4-({6-[(6-chloro-3-{1-[(4-chlorophenyl)methyl]-4-(4-fluorophenyl)-1H-imidazol-5-yl}-1H-indole-2-carbonyl)oxy]hexyl}amino)-4-oxobutanoic acid | C35 H33 Cl2 F N4 O5 | 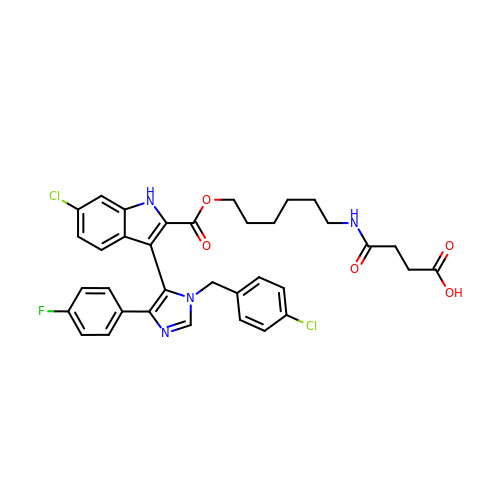MEJMFPQUMDEAQP-UHFFFAOYSA-N N-({3-hydroxy-2-methyl-5-[(phosphonooxy)methyl]pyridin-4-yl}methyl)-L-methionine | C13 H21 N2 O7 P S | 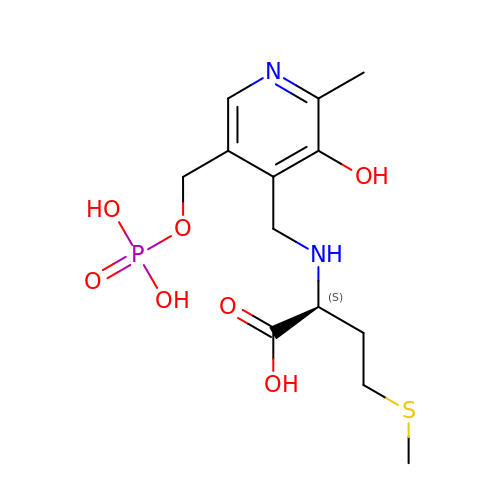TZGVKKRKUOYYOG-NSHDSACASA-N> MLQQVFGKSKGGEVTNSHLTPKVLNKAQEAEKLASQIQAQRFSNRLVAFSSQYPRAKLFFAGIGIGTLLYGANQSSKARENKVATETRKERMAKPTIQLTGADSQNPPFTEKNINDWLYKTVSITGRPIHGKGMMIPAKSYGLHGFEYLVPFVTKENEDGSVQEGLILNLGFIPREYAPIWARARVENVEEQTFTCVVTDGKHLSEQGG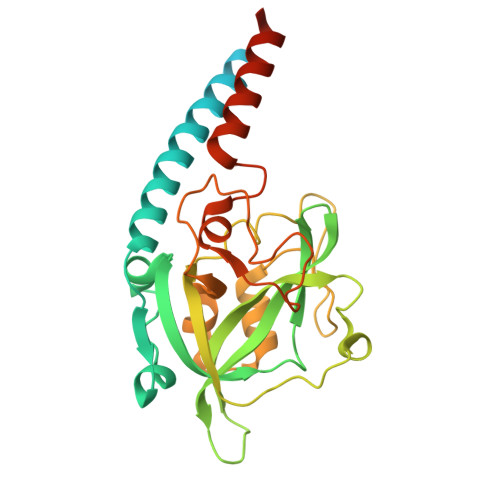LFASNKPCENQWEYADLDQLAKHTGFVNQEQVRSCILEHVNTETPNDERDCRHIDICSDYKEDYPYKFTRSGVLQQPGQMYWDLNKSASYYSLLGLGCSVFSALLFLAK> GHMLFGVKCHNTDSEPLKNEDLLKNLLTMGVDIDMARKRQPGVFHRMITNEQDLKMFLLSKGASKEVIASIISRYPRAITRTPENLSKRWDLWRKIVTSDLEIVNILEASPESFFRSNNNLNLENNIKFLYSVGLTRKCLCRLLTNAPRTFSNSLDLNKQMVEFLQAAGLSLGHNDPADFVRKIIFKNPAILIQSTKRVKANIEFLRSTFNLNSEELLVLICGPGAEILDLSNDAARRSYANIKEKLFSLGCTEEEVQKFVLSYPDVIFLAEKKFNDKIDCLMEENISISQIIENPR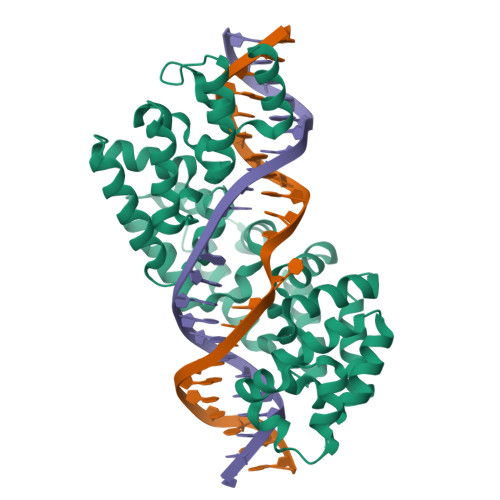VLDSSISTLKSRIKELVNAGCNLSTLNITLLSWSKKRYEAKLKKLS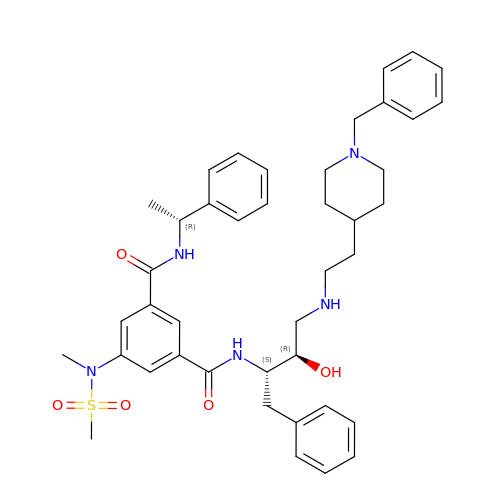N-[(2S,3R)-4-{[2-(1-benzylpiperidin-4-yl)ethyl]amino}-3-hydroxy-1-phenylbutan-2-yl]-5-[methyl(methylsulfonyl)amino]-N'-[(1R)-1-phenylethyl]benzene-1,3-dicarboxamide | C42 H53 N5 O5 S | IMNAYTZSJCRZIO-RLRCJDGOSA-N> VEWTDFERATIKDIFSKLEYDVVGPATLARCLVVYPWTQR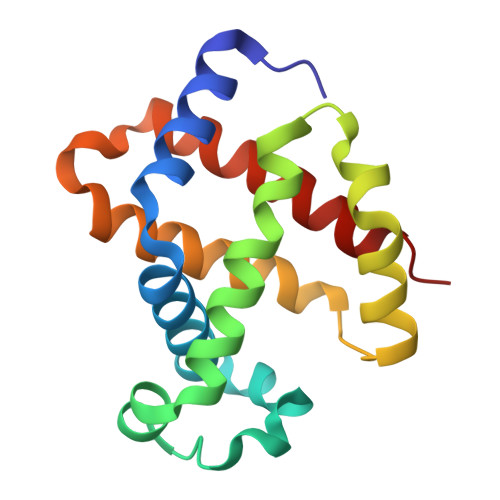YFGKFGNLYNAAAIAQNAMVSKHGTTILNGLDRAVKNMDDITNTYAELSVLHSEKLHVDPDNFKLLADCLTIVVAARFGSAFTGEVQAAFQKFMAVVVSSLGKQYR>[4x]MDKFRIQGSDKPLSGEVTI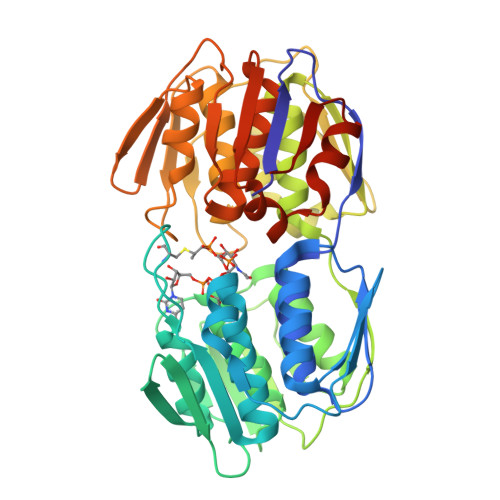SGAKNAALPILFASLLAEEPVEVANVPKLRDVDTTMELLKRLGAEVSRNGSVHIDASGVNDFCAPYDLVKTMRASIWALGPLVARFGKGQVSLPGGCAIGARPVDLHIHGLEQLGATIKLEEGYVKAEVDGRLKGAHIVMDKVSVGATITVMCAATLAEGTTVLENAAREPEIVDTANFLNAIGAKVSGMGTDTITIEGVERLGGGYHEVVADRIETGTFLVAAAVSGGKIVCKNTKAHLLEAVLAKLEEAGADVQTGDDWISLDMTGRELKAVNIRTAPHPAFPTDMQAQFTLLNMMAKGSGIITETIFENRFMHIPELQRMGAHAEIEGNTAICGDTDGLSGAQVMATDLRASASLVIAGCIAKGETIVDRIYHIDRGYDKIEDKLTALGANIERVHSDDLLEHHHHHH>[3x]GPPTSDDIFEREYKYGAHNYHPLPVALERGKGIYLWDVEGRKYFDFLSSYSAVNQGHCHPKIVNALKSQ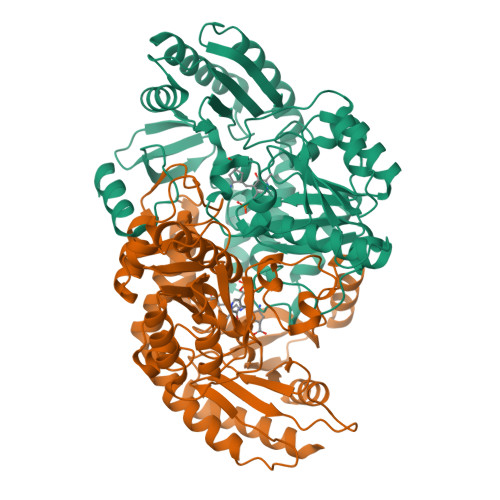VDKLTLTSRAFYNNVLGEYEEYITKLFNYHKVLPMNTGVEAGETACKLARKWGYTVKGIQKYKAKIVFAAGNFWGRTLSAISSSTDPTSYDGFGPFMPGFDIIPYNDLPALERALQDPNVAAFMVEPIQGEAGVVVPDPGYLMGVRELCTRHQVLFIADEIQTGLARTGRWLAVDYENVRPDIVLLGKALSGGLYPVSAVLCDDDIMLTIKPGEHGSTYGGNPLGCRVAIAALEVLEEENLAENADKLGIILRNELMKLPSDVVTAVRGKGLLNAIVIKETKDWDAWKVCLRLRDNGLLAKPTHGDIIRFAPPLVIKEDELRESIEIINKTILSF>[2x]MAHHHHHHMADWVSGKVTKVEYWTDALFSLYVRAPVHPFTAGQFTKLGLEIDGERVQRAYSYVNAPGNPDLEFYLVTVPEGKLSPRLASLKPGDEVLVVSEAAGFFVLEEVP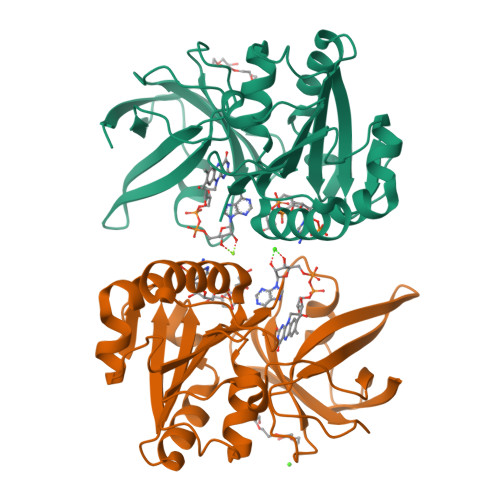DCDTLWMLATGTALGPYLSILQEGKDLERFNNLVLVHAVRYAADLSYLPLMRELEQRYAGKLRIQTVVSRETVEGSLTGRVPFLIETGALEEAVGLPMTTDTSHVMLCGNPQMVRDTQQLLKETRQMTKHLRRRPGHMTAEHYW(2~{R})-~{N}-(2,2-dimethylpropyl)-1-[4-(4-ethanoyl-3-ethyl-5-methyl-1~{H}-pyrrol-2-yl)-1,3-thiazol-2-yl]piperazine-2-carboxamide | 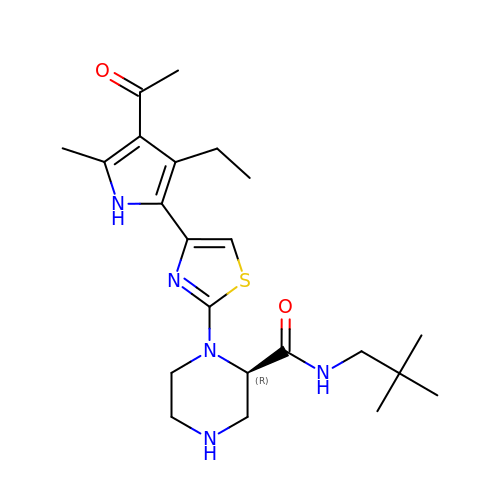C22 H33 N5 O2 S | BIQUDHDFGPBAHX-QGZVFWFLSA-N> TIQPGTGYNNGYFYSYWNDGHGGVTYTNGPGGQFSVNWSNSGEFVGGKGWQPGTKNKVINFSGSYNPNGNSYLSVYGWSRNPLIEYYIVENFGTYNPSTGATKLGEVTS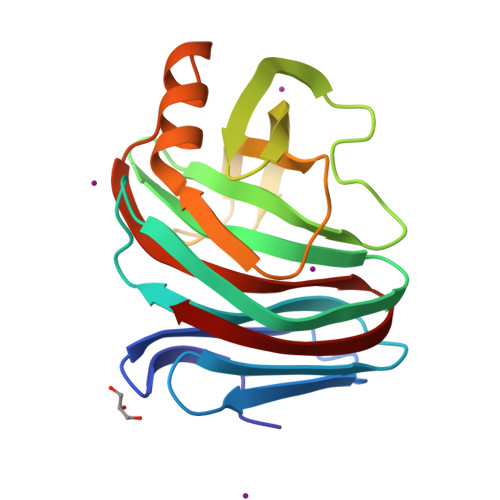DGSVYDIYRTQRVNQPSIIGTATFYQYWSVRRNHRSSGSVNTANHFNAWAQQGLTLGTMDYQIVAVNGYFSSGSASITVS5-({4-[(1R,4S)-3'-methyl[1,2,3,4-tetrahydro[1,1'-biphenyl]]-4-yl]piperazin-1-yl}methyl)pyridin-2(1H)-one 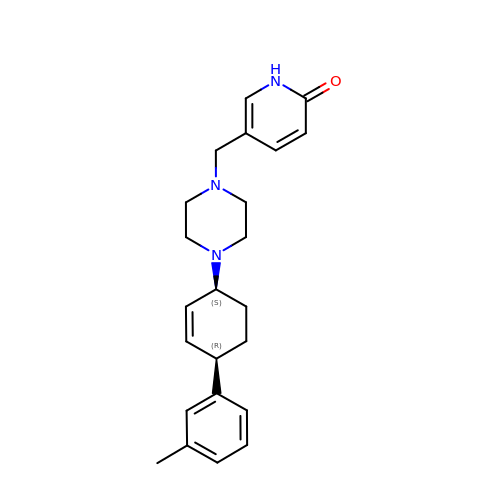| C23 H29 N3 O | FHCQTFCSGMYNPX-RBBKRZOGSA-N In contrast to its eukaryotic counterparts, bacterial HSS synthesizes 1 mol HSP from 2 mol PUT. NAD+ serves as a non-covalently bound prosthetic group for BvHSS. The interface area of the dimer was calculated as approximately 1700 Å2 by PDBsum indicating a stable dimer23. The BvHSS subunit consists of two domains as determined by CATH24: one “NAD(P)-binding Rossmann-like” domain (domain 1, residues 3–163 and 394–425) and one “homospermidine-synthase-like domain” (domain 2, residues 164–395 and 426–477) as shown in Fig. 2a and S1. The crystal structures of BvHSS containing NAD+ clearly show that the active site is localized inside each subunit.

1,3-Diaminopropane (DAP) is the only known diamine functioning as a strong competitive inhibitor of bacterial HSS910. The innermost nitrogen ND of the DAP at the active site is coordinated to Asn-162 and oxygen O7N of NAD+ , whereas nitrogen NAA is coordinated to Glu-237 and oxygen O2D of NAD+ . With the nitrogen NAA position being found near the inner amino site and the nitrogen ND position being found near the center amino site (shifted towards the inner amino site), the overall geometry of DAP has to be slightly “stretched” to fit the observed electron density. The innermost nitrogen ND of the second DAP is coordinated to Glu-117 and oxygen O2D of NAD+ , whereas nitrogen NAA is coordinated to Ser-236 and oxygen O of Glu-232. Thus, the nitrogen ND is positioned at the proposed ionic interaction site 2 of the “ionic slide” (refer to Fig. 2d). The other nitrogen is positioned slightly “below” the proposed ionic interaction site 1. In case of a PUT instead of a DAP, the corresponding nitrogen would still be positioned slightly below the ionic interaction site 1. This supports the proposed function of the ionic slide as being a substrate guiding mechanism: The observed electron density of this second DAP appears well defined and is not “smeared” as in the case of the first DAP. In contrast to PUT, neither DAP nor CAD have been detected either at a distinct position at the inner binding site or at the outer binding site in HSS crystal structures. Instead, only DAP is found to swap potentially between the inner and outer sites without being oxidized. Thus, DAP can compete against PUT for both binding sites explaining its reported competitive inhibitory effect.

>[2x]DWPVYHRIDGPIVMIGFGSIGRGTLPLIERHFAFDRSKLVVIDPSDEARKLAEARGVRFIQQAVTRDNYRELLVPLLTAGPGQGFCVNLSVDTSSLDIMELARENGALYIDTVVEPWLGFYFDPDLKPEARSNYALRETVLAARRNKPGGTTAVSCCGANPGMVSWFVKQALVNLAADLGVTGEEPTTREEWARLAMDLGVKGIHIAERDTQRASFPKPFDVFVNTWSVEGFVSEGLQPAELGWGTFERWMPDNARGHDSGCGAGIYLLQPGANTRVRSWTPTAMAQYGFLVTHNESISIADFLTVRDAAGQAVYRPTCHYAYHPCNDAVLSLHEMFGSGKRQSDWRILDETEIVDGIDELGVLLYGHGKNAYWYGSQLSIEETRRIAPDQNATGLQVSSAVLAGMVWALENPNAGIVEADDLDFRRCLEVQTPYLGPVVGVYTDWTPLAGRPGLFPEDIDTSDPWQFRNVLVRD>[2x]MRGLAVLVLLVFAVQVAAAE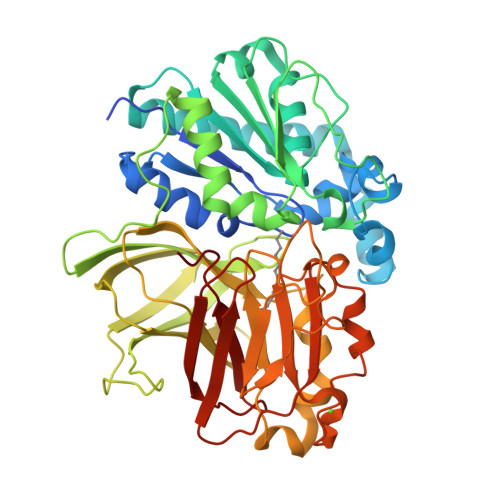DFRPVVFVHGLAGSAGQFESQGMRFAANGYPAEYVKTFEYDTISWALVVETDMLFSGLGSEFGLNISQIIDPETLDKILSKSRERLIDETFSRLDRVIDEALAESGADKVDLVGHAMGTFFLVRYVNSSPERAAKVAHLILLDGVWGVDAPEGIPTLAVFGNPKALPALGLPEEKVVYNATNVYFNNMTHVQLCTSPETFAVMFEFINGYKPATTDIVPQDGDYVKVKGKFLAFATNGDVSGWLSIYPIDENGKRLTRLPVKFMRVKGDFEVRLRKGQLYEFQFRKDFSPIIYHYYRAPFVRDDLWARFLVSKPPLDVELLILPERLSPAAKETSGLLLIRYKEMIGEYDEEIGGVDEVYVNGVNVCTERICPIERAVNGLWVFDRGADGKSDLDREVVRYSIMPFMSAADLVVPAEGTISIAVKSRTGGEESFTIPAWSADRHSIIVQFSDYIV> G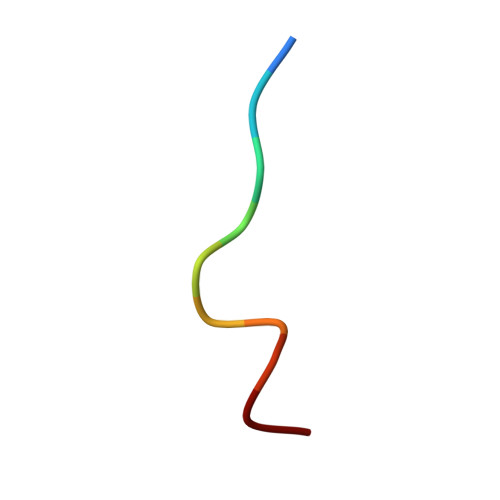YENPTYKFF N-(1,3-thiazol-2-yl)quinoxaline-6-carboxamide | C12 H8 N4 O S | 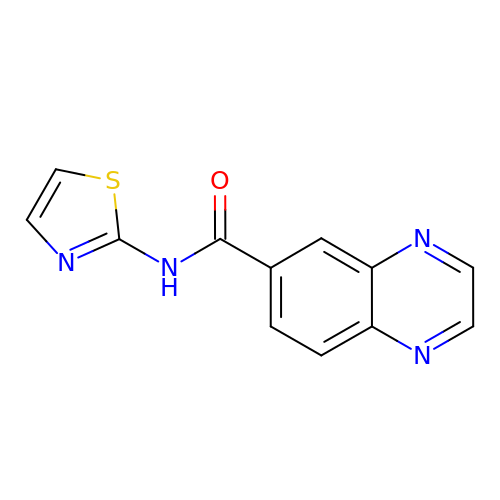GKTOUDJRQSWCBO-UHFFFAOYSA-N> GMSEENKIGTYQFVAEPFHVDFNGRLTMGVLGNHLLNCAGFHASDRGFGIATLNEDNYTWVLSRLAIELDEMPYQYEKFSVQTWVENVYRL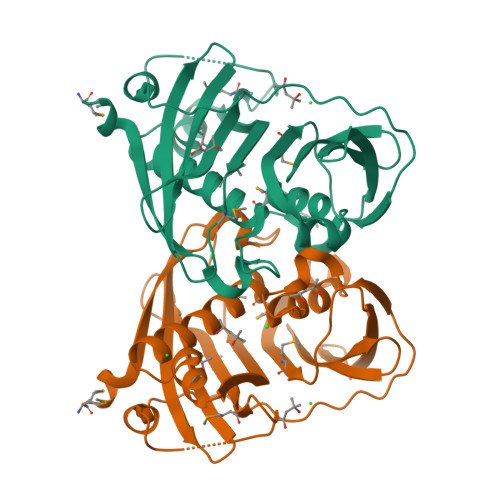FTDRNFAVIDKDGKKIGYARSVWAMINLNTRKPADLLALHGGSIVDYICDEPCPIEKPSRIKVTSNQPVATLTAKYSDIDINGHVNSIRYIEHILDLFPIELYQTKRIRRFEMAYVAESYFGDELSFFCDEVSENEFHVEVKKNGSEVVCRSKVIFE>[2x]MESLPVIAAPSMWTRPQIRDFKEKIRQDSDSVITVGRGEVVTVRVPTHEEGSYLFWEFATDNYDIGFGVYFEWTDSPNTAVSVHVSESSEHDD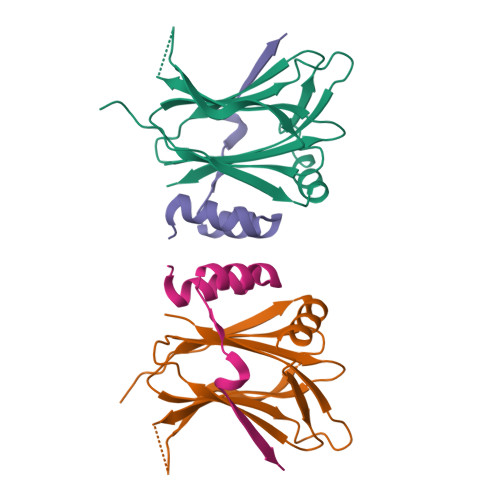EEEEENISSEEKAKKNANKPVLDEIVPVYRRDCHEEVYAGSHQYPGRGVYLLKFDNSYSLWRSKSVYYRVYYTR;>GPPQFKPLKISVDPEIPAPPAIADLLASVDSEEVREYCKKKGWIVEVPVTATTLERNVS[2x]3-chloro-N-(4-morpholin-4-ylphenyl)-6-pyridin-3-ylimidazo[1,2-a]pyrazin-8-amine 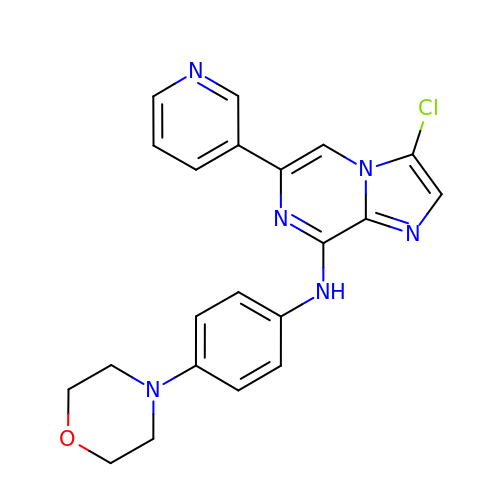| C21 H19 Cl N6 O | FXFAGYZXIGMEEG-UHFFFAOYSA-N> MFKIGSVLKQIRQELNYHQIDLYSGIMSKSVYIKVEADSRPISVEELSKFSERLGVNFFEILNRAGMNTKSVNETGKEKLLISKIFTNPDLFDKNFQRIEPKRLTSLQYFSIYLGYISIAHHYNIEVPTFNKTITSDLKHLYDKRTTFFGIDYEIVSNLLNVLPYEEVSSIIKPMYPIVDSFGKDYDLTIQTVLKNALTISIMNRNLKEAQYYINQFEHLKTIKNISINGYYDLEINYLKQIYQFLTDKNIDSYLNAV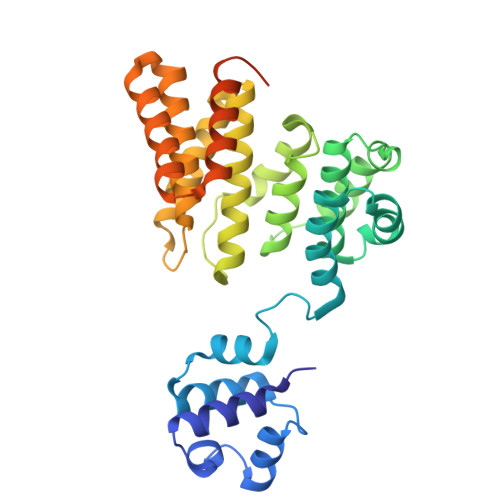NIINIFKIIGKEDIHRSLVEELTKISAKEKFTPPKEVTMYYENYVAIENNPIPEIKEQS(TERT-BUTYLOXYCARBONYL)-ALANYL-AMINO 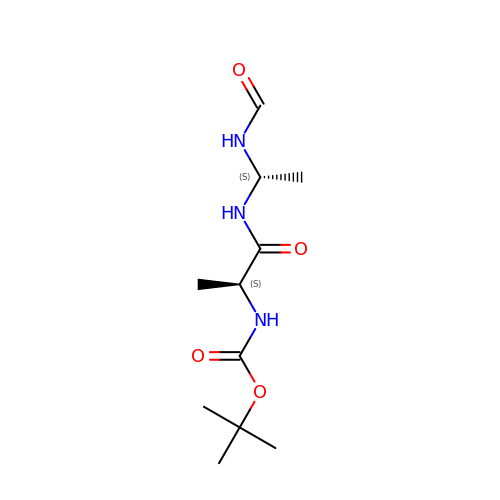ETHYL-FORMAMIDE | C11 H21 N3 O4 | MNUWNIQGBRBQRE-YUMQZZPRSA-N> MSALFEPYTLKDVTLRNRIAIPPMCQYMAEDGMINDWHHVHLAGLARGGAGLLVVEATAVAPEGRITPGCAGIWSDAHAQAFVPVVQAIKAAGSVPGIQIAHAGRKASANRPWEGDDHIAADDTRGW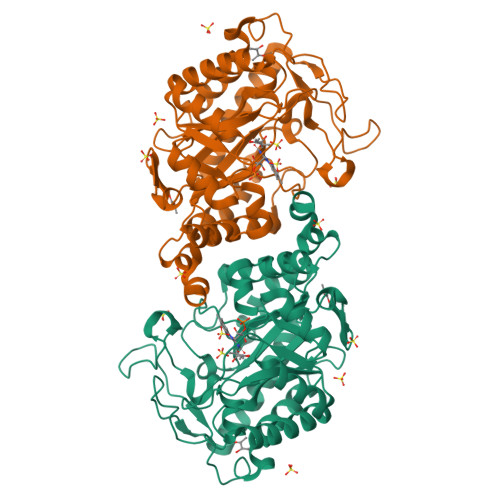ETIAPSAIAFGAHLPKVPREMTLDDIARVKQDFVDAARRARDAGFEWIELHFAHGYLGQSFFSEHSNKRTDAYGGSFDNRSRFLLETLAAVREVWPENLPLTARFGVLEYDGRDEQTLEESIELARRFKAGGLDLLSVSVGFTIPDTNIPWGPAFMGPIAERVRREAKLPVTSAWGFGTPQLAEAALQANQLDLVSVGRAHLADPHWAYFAAKELGVEKASWTLPAPYAHWLERYR R2 elements, a class of non-long terminal repeat (non-LTR) retrotransposons, have the potential to be harnessed for transgene insertion. To insert a new copy of itself, the R2 protein recruits the R2 RNA and nicks the bottom strand of the 28S DNA. Using the nicked DNA as a primer and the R2 RNA as a template, it reverse transcribes a new copy of the element – a process known as target-primed reverse transcription (TPRT). The R2Tg element is a member of the R2-A clade common in birds, with several differences compared to R2Bm, which is in the R2-D clade.

To understand differences in the DNA and RNA-binding properties of R2Tg and R2Bm, we incubated R2Tg protein with a biotinylated DNA substrate and 149 nt of 3′ UTR RNA + 40 nt of 3′ homology in the presence of dideoxythymidine to stall TPRT after reverse transcription of a single nucleotide. We purified stalled TPRT complexes using streptavidin beads and solved their structure by cryo-EM to 3.2 Å resolution. The nicked bottom strand is annealed to the RNA 3′ homology within the RT domain, and the 3′ UTR is bound by the RT − 1 domain. In the 325-nt R2Tg 3′ UTR, we similarly found two double-stranded regions with a single-stranded linker, but these were contiguous in sequence space, directly forming the 3′ 67 nt of the 3′ UTR, consistent with our TPRT assays on truncated substrates. The first of these double-stranded regions, equivalent to P1 in R2Bm, forms a pseudoknot with three base triples, resulting in the ordered region of the R2Tg 3′ UTR being larger and more extensive than the R2Bm 3′ UTR. The Myb domain, which binds the start of the RUM in R2Bm, was not resolved in our cryo-EM density despite being present in our expression construct. The ZnF domain in common with R2Bm (ZnF 1) inserts an alpha helix into the minor groove of the target DNA, similar to R2Bm, but forms hydrogen bonds to different bases. Therefore, although R2Tg and R2Bm bind to the same DNA substrate with similar DNA-binding domains, they read out different bases of the target using different residues from the same domains. The two additional N-terminal ZnF domains in R2Tg, characteristic of the R2-A clade of R2 elements, were not immediately apparent in our cryo-EM density. However, after low-pass filtering we were able to dock AlphaFold models of these domains above the minor groove of the target DNA between positions –12 to –9.

> MASCPKPGPPVSAGAMSLESGLTTHSVLAIERGPNSLANSGSDFGGGGLGLPLRLLRVSVGTQTSRSDWVDLVSWSHPGPTSKSQQVDLVSLFPKHRVDLLSKNDQVDLVAQFLPSKFPPNLAENDLALLVNLEFYRSDLHVYECVHFAAHWEGLSGLPEVYEQLAPQPCVGETLHSSLPRDSELFVPEEGSSEKESEDAPKTSPPTPGKHGLEQTGEEKVMVTVPDKNPPCPCCGTRVNSVLNLIEHLKVSHGKRGVCFRCAKCGKENSNYHSVVCHFPKCRGPETEKAPAGEWICEVCNRDFTTKIGLGQHKRLAHPAVRNQERIVASQPKETSNRGAHKRCWTKEEEELLIRLEAQFEGNKNINKLIAEHITTKTAKQISDKRRLLSRKPAEEPREEPGTCHHTRRAAASLRTEPEMSHHAQAEDRDNGPGRRPLPGRAAAGGRTMDEIRRHPDKGNGQQRPTKQKSEEQLQAYYKKTLEERLSAGALNTFPRAFKQVMEGRDIKLVINQTAQDCFGCLESISQIRTATRDKKDTVTREKHPKKPFQKWMKDRAIKKGNYLRFQRLFYLDRGKLAKIILDDIECLSCDIPLSEIYSVFKTRWETTGSFKSLGDFKTYGKADNTAFRELITAKEIEKNVQEMSKGSAPGPDGITLGDVVKMDPEFSRTMEIFNLWLTTGKIPDMVRGCRTVLIPKSSKPDRLKDINNWRPITIGSILLRLFSRIVTARLSKACPLNPRQRGFIRAAGCSENLKLLQTIIWSAKREHRPLGVVFVDIAKAFDTVSHQHIIHALQQREVDPHIVGLVSNMYENISTYITTKRNTHTDKIQIRVGVKQGDPMSPLLFNLAMDPLLCKLEESGKGYHRGQSSITAMAFADDLVLLSDSWENMNTNISILETFCNLTGLKTQGQKCHGFYIKPTKDSYTINDCAAWTINGTPLNMIDPGESEKYLGLQFDPWIGIARSGLSTKLDFWLQRIDQAPLKPLQKTDILKTYTIPRLIYIADHSEVKTALLETLDQKIRTAVKEWLHLPPCTCDAILYSSTRDGGLGITKLAGLIPSVQARRLHRIAQSSDDTMKCFMEKEKMEQLHKKLWIQAGGDRENIPSIWEAPPSSEPPNNVSTNSEWEAPTQKDKFPKPCNWRKNEFKKWTKLASQGRGIVNFERDKISNHWIQYYRRIPHRKLLTALQLRANVYPTREFLARGRQDQYIKACRHCDADIESCAHIIGNCPVTQDARIKRHNYICELLLEEAKKKDWVVFKEPHIRDSNKELYKPDLIFVKDARALVVDVTVRYEAAKSSLEEAAAEKVRKYKHLETEVRHLTNAKDVTFVGFPLGARGKWHQDNFKLLTELGLSKSRQVKMAETFSTVALFSSVDIVHMFASRARKSMVM> MLPQRLHPSRLLALALFSLVL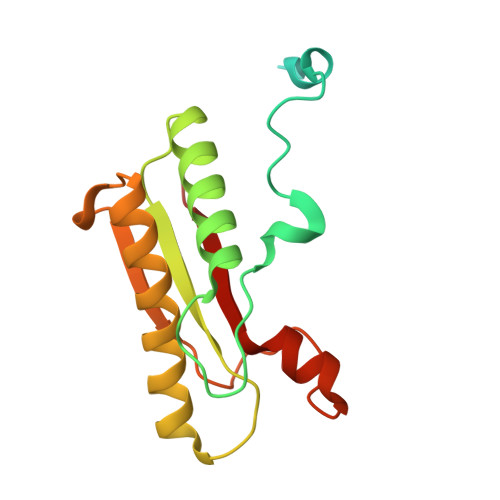GLAGCQTKPPQTGLSAEQIAVPQEQGFELRDEGWEFGMSSKVLFGNNLDRLNPDSRNTLTKIARALLAVDIDKVRLEGHTDNYGDEGYNQKLSERRAESVAAVFREAGMPAANIEVRGLGMSKPVADNKTRAGRSENRRVAIIVPAE>SNAMSGMRFGTRLVHGGRRPSAGTGDVVPPIHVSTTYERRAQDEPRYFYGRGENPTREELEECLAGLERAPFATVFSSGQAAAATLLSLVRPGQCVVSTDDVYAGTDGLFDLAARQGVRVRYADLTTPEGIAAALAEPDLALVWIETPTNPLLTVVDVAEVSRRAHERGARVVVDNTFASPVLQQPLALGADVSLYSTTKSIAGHADVLGGALVYRDADLHAAVRAYRTTAGNVPGALDCFLVRRGLHTLSLRVHRQVATARVLVERLRASPVVGAVHYPGLPEHPQHAVVKAQMSAPGAIVSFDYLGGPAERLLDRFTLFTCGVSLGGVHSLVECPALMTHRPLSAEARARRGIGESLIRLSVGIEDPQDLAEDLSRALAGGT[8x]

We have applied ENM and ensemble refinement approaches to extract the dynamic information from the experimental structure of CalE6, a PLP (pyridoxal 5′ phosphate)-dependent methionine γ-lyase from Micromonospora echinospora, which is encoded by the calicheamicin biosynthetic gene cluster. Calicheamicin γ1I is a prototype of the 10-membered enediyne family of antibiotics that contains a characteristic bicyclo[7.3.1]tridecadiynene core. Among the putative genes responsible for sulfur transfer during calicheamicin biosynthesis, the corresponding gene product CalE6 was recently confirmed to show methionine γ lyase activity. However, the contribution of this enzymatic activity to calicheamicin thiosugar and/or trisulfide formation remains unknown.

The crystal structure of CalE6 was determined and refined to a resolution of 2.1 Å. Two homotetramers were found in the asymmetric unit displaying essentially the same conformational state with overall Cα RMSD of 0.143 over 1509 residues of four chains (A–D vs. E–F). Each tetramer harbors four molecules of PLP, each bound in a cleft formed at C-2 symmetry-related dimer interfaces. Within the dimer, one subunit provides Lys 197 as the Schiff-base anchor for PLP and forms multiple non-covalent interactions with the cofactor from residues Ser 75, Gln 77, Tyr 100, Glu 143, Asp 172, Thr 174, Ser 194, Thr 196. The adjacent subunit provides additional charge-charge and hydrogen-bonding interactions with the phosphate group of PLP from residues Arg 48′ and Tyr 46′ located on an extended loop (residues 14–51). Despite little structural difference between the two ligand bound forms, all four subunits consistently showed nontrivial local conformational changes involving ∼17° side-chain rotation of the active site residue Tyr 100, a highly conserved residue structurally stacking with the pyridine ring of the cofactor in PLP-dependent enzymes. The major movement of Tyr 100 involves rotation around Cβ-Cγ bond with minor shift of backbone positions resulting in a 16.5° decrease of Cα-Cβ-Cγ-Cδ1 dihedral angle from 67.4 ± 0.7° to 50.9 ± 2.4°. Ngo et al. have proposed that the catalytic cycle of PLP-dependent enzymes may actively involve PLP conformational changes upon formation of external aldimine as observed in Xanthomonas oryzae cystathionine γ-lyase. This PLP conformational change was not observed in the CalE6-MES complex likely because the substrate mimic, lacking the α-amino group, is unable to form the external aldimine linkage with PLP. We further simulated the dynamics and sampled the conformational space of this enzyme using both coarse-grain elastic network models and ensemble refinement methods based on the CalE6-MES complex structure. Ensemble refinement was able to identify the different rotamers of Tyr 100 of CalE6 covering the conformational space as observed in the static crystal structures of different ligand complexes (MES vs. sulfate).(2E,4S,5R,6R,7S,8R)-5-(acetylamino)-4,6,7,8,9-pentahydroxy-2-(hydroxyimino)nonanoic acid (non-preferred 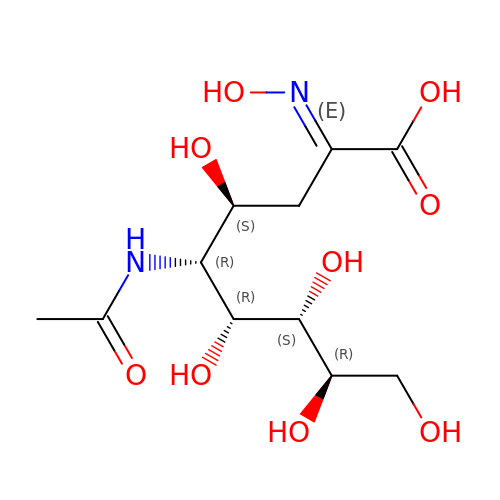name) | C11 H20 N2 O9 | ROZSOFSDDJZICT-HMLDMLNFSA-N> MGSEESNNICAYKRTISLAKIYIVLLVKTAMLRYSRLCFPKMGCEEITRKARRVQLQ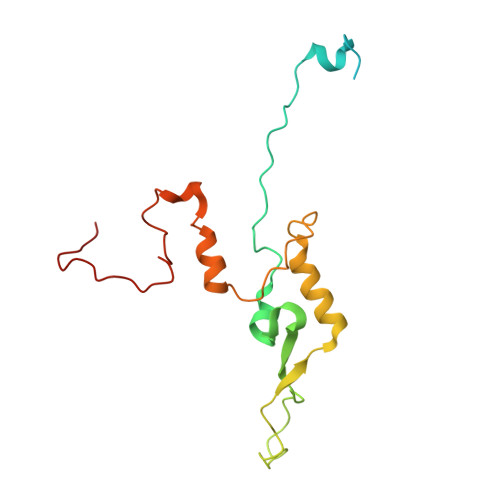PTEYLAQHRMQVWQLRFKEMGPPFSRVWVALGGKMRRRRVGRQVDVKDMRYYWRPIEPQYQRLYMSRLRIRDHSNKLRQPMRLRATNADIGSGSSSIEWERASNRKYGAMLAPPKRQDFEFRVV2-[1-(4-chlorobenzene-1-carbonyl)-5-methoxy-2-methyl-1H-indol-3-yl]-N-[4-({[5-(dimethylamino)naphthalen-1-yl]sulfonyl}amino)butyl]acetamide 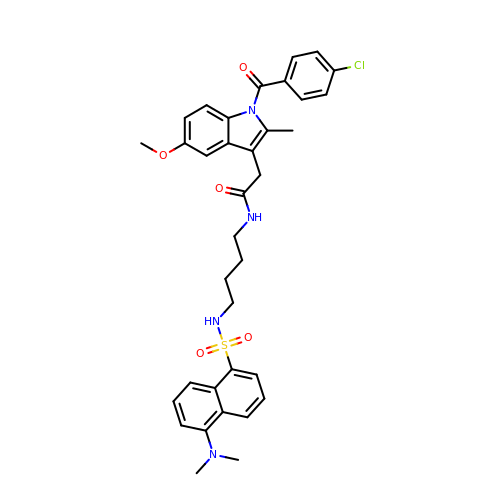| C35 H37 Cl N4 O5 S | YGEBTZVDTLWCOG-UHFFFAOYSA-N Jingmenviruses are a category of emerging segmented viruses that have garnered global attention in recent years, and are close relatives of the flaviviruses in the Flaviviridae family. One of their genome segments encodes NSP1 homologous to flavivirus NS5. NSP1 comprises both the methyltransferase (MTase) and RNA-dependent RNA polymerase (RdRP) modules playing essential roles in viral genome replication and capping. The NSP1 RdRP exhibits a characteristic architectural feature commonly found in viral RdRPs, known as encircled right-hand architecture.

To gain insights into the structural characteristics of jingmenvirus NSP1, we conducted a crystallization screening experiment for three variants: FL (residues 1–915) JMTV NSP1, as well as two N-terminal truncation constructs, namely D55 (residues 56–915) and D307 (residues 308–915). Although the FL construct did not yield any crystals, the D55 and D307 constructs produced crystals with flake-like and stick-like shapes, respectively. The initial determination of the structure of D55 involved the utilization of the SAD method, wherein Se-Met-substituted D55 crystals were employed. Subsequently, the structures of native D55 and D307 were resolved through molecular replacement, utilizing the Se-Met-derived D55 structure as the search model. The D55 crystal was found to be an N-terminal degraded D55 protein, but the precise N-terminus of the protein in the crystal was not determined. However, electron density was not detected for residues 56–302 in both the native and Set-Met-derived D55 structures. All three structures are isomorphous with the same P212121 space group cell dimensions. Each crystallographic asymmetric unit consists of a single NSP1 monomer. Due to the significant similarity between the native structures of D55 and D307, with a root-mean-square deviation (RMSD) value of merely 0.2 Å for all superimposable α-carbon atoms (with D307 structure as the reference, covering 99.5% of residues), we primarily utilize the 1.84-Å D307 structure for subsequent illustrations.

> MEPTLGDPTELGRQAKKEMNAMTYEEFDRMKFRGVVAEVYAGDKPSKGYDKLRTLLDLMDRPKLGTTVDLCAGRGGWSQLVGELEGPGDITAVSLWERGREEWMADPAIRRINANVKNVKPWRVDTLLFDGGETFKRDQNIMKEESYNDALLDAVDAWMMQATPPTNFVIKIQVPYTQKAMRLIEKWQVKTKKGRLVRLAGDRLSNTVMYFISDRLETQIRGRITSFLRELRERRVDRSLTSDPALQYERITPEWTAEAVIEGCAPLTPLNMTRSIAEMHMEYPPLGITRFFKELGYKIAKKKGSEGTRKNRFVGQLIEPLRRVLERHHLFGAWQLTSTTPRAVFNMFRSKVDRAPVELHSHYPGLKKMYDILADLWLERYGSMKRLTEEEMASAINRRGAMGYQMDNRNYGDLGAYWDSGDWRQDVNTFKRALLSGTPTHAVYNTTAKKEKTKNLTRQVNKGSRIIQYLPADARLYELKVLGGLHKYLEKCGWSVAGQGLYKYGDRVKKSMDATGAAISEDVAGWDTKISKGLLTLESHMFTKLAEDEEMAREIHHLYRLYADPHMVVQREIEGEVHDVLLRGRGQVSSGRQPTYAANTITNFITTTYGMAVTLGIPEADWPRLIRDLTDERGNRRLLVSGDDKVLFLRGDEARVYASSAYRISNDMGLVRKDMALEQESEIIVDVKEISFCSHRYWPVKYGNEIHYMPVRDVGEIFAKATMALGVYKDDMTQEAWARVQGLNMLVNYHHIPECRMLALAILSVTRIGLNLKGITKGWMMSTEWLRDDLAPDTIHALITEGRTSGWDQLGYVDFKDRKGILLRPDTNYKNWRRDLPEKVRQLREDGQYKDWLQKMAVFGGSSSGTHHHHHH>MDYKDDDDKLAAANSSIDLISTSLYKKAGFRTMTSIHFVVHPLPGTEDQLNDRLREVSEKLNKYNLNSHPPLNVLEQATIKQCVVGPNHAAFLLEDGRVCRIGFSVQPDRLELGKPDNNDGSKLNSNSGAGRTSRPGRTSDSPWFLSGSETLGRLAGNTLGSRWSSGVGGSGGGSSGRSSAGARDSRRQTRVIRTGRDRGSGLLGSQPQPVIPASVIPEELISQAQVVLQGKSRSVIIRELQRTNLDVNLAVNNLLSRDDEDGDDGDDTASESYLPGEDLMSLLDADIHSAHPSVIIDADAMFSEDISYFGYPSFRRSSLSRLGSSRVLLLPLERDSELLRERESVLRLRERRWLDGASFDNERGSTSKEGEPNLDKKNTPVQSPVSLGEDLQWWPDKDGTKFICIGALYSELLAVSSKGELYQWKWSESEPYRNAQNPSLHHPRATFLGLTNEKIVLLSANSIRATVATENNKVATWVDETLSSVASKLEHTAQTYSELQGERIVSLHCCALYTCAQLENSLYWWGVVPFSQRKKMLEKARAKNKKPKSSAGISSMPNITVGTQVCLRNNPLYHAGAVAFSISAGIPKVGVLMESVWNMNDSCRFQLRSPESLKNMEKASKTTEAKPESKQEPVKTEMGPPPSPASTCSDASSIASSASMPYKRRRSTPAPKEEEKVNEEQWSLREVVFVEDVKNVPVGKVLKVDGAYVAVKFPGTSSNTNCQNSSGPDADPSSLLQDCRLLRIDELQVVKTGGTPKVPDCFQRTPKKLCIPEKTEILAVNVDSKGVHAVLKTGNWVRYCIFDLATGKAEQENNFPTSSIAFLGQNERNVAIFTAGQESPIILRDGNGTIYPMAKDCMGGIRDPDWLDLPPISSLGMGVHSLINLPANSTIKKKAAVIIMAVEKQTLMQHILRCDYEACRQYLMNLEQAVVLEQNLQMLQTFISHRCDGNRNILHACVSVCFPTSNKETKEEEEAERSERNTFAERLSAVEAIANAISVVSSNGPGNRAGSSSSRSLRLREMMRRSLRAAGLGRHEAGASSSDHQDPVSPPIAPPSWVPDPPAMDPDGDIDFILAPAVGSLTTAATGTGQGPSTSTIPGPSTEPSVVESKDRKANAHFILKLLCDSVVLQPYLRELLSAKDARGMTPFMSAVSGRAYPAAITILETAQKIAKAEISSSEKEEDVFMGMVCPSGTNPDDSPLYVLCCNDTCSFTWTGAEHINQDIFECRTCGLLESLCCCTECARVCHKGHDCKLKRTSPTAYCDCWEKCKCKTLIAGQKSARLDLLYRLLTATNLVTLPNSRGEHLLLFLVQTVARQTVEHCQYRPPRIREDRNRKTASPEDSDMPDHDLEPPRFAQLALERVLQDWNALKSMIMFGSQENKDPLSASSRIGHLLPEEQVYLNQQSGTIRLDCFTHCLIVKCTADILLLDTLLGTLVKELQNKYTPGRREEAIAVTMRFLRSVARVFVILSVEMASSKKKNNFIPQPIGKCKRVFQALLPYAVEELCNVAESLIVPVRMGIARPTAPFTLASTSIDAMQGSEELFSVEPLPPRPSSDQSSSSSQSQSSYIIRNPQQRRISQSQPVRGRDEEQDDIVSADVEEVEVVEGVAGEEDHHDEQEEHGEENAEAEGQHDEHDEDGSDMELDLLAAAETESDSESNHSNQDNASGRRSVVTAATAGSEAGASSVPAFFSEDDSQSNDSSDSDSSSSQSDDIEQETFMLDEPLERTTNSSHANGAAQAPRSMQWAVRNTQHQRAASTAPSSTSTPAASSAGLIYIDPSNLRRSGTISTSAAAAAAALEASNASSYLTSASSLARAYSIVIRQISDLMGLIPKYNHLVYSQIPAAVKLTYQDAVNLQNYVEEKLIPTWNWMVSIMDSTEAQLRYGSALASAGDPGHPNHPLHASQNSARRERMTAREEASLRTLEGRRRATLLSARQGMMSARGDFLNYALSLMRSHNDEHSDVLPVLDVCSLKHVAYVFQALIYWIKAMNQQTTLDTPQLERKRTRELLELGIDNEDSEHENDDDTNQSATLNDKDDDSLPAETGQNHPFFRRSDSMTFLGCIPPNPFEVPLAEAIPLADQPHLLQPNARKEDLFGRPSQGLYSSSASSGKCLMEVTVDRNCLEVLPTKMSYAANLKNVMNMQNRQKKEGEEQPVLPEETESSKPGPSAHDLAAQLKSSLLAEIGLTESEGPPLTSFRPQCSFMGMVISHDMLLGRWRLSLELFGRVFMEDVGAEPGSILTELGGFEVKESKFRREMEKLRNQQSRDLSLEVDRDRDLLIQQTMRQLNNHFGRRCATTPMAVHRVKVTFKDEPGEGSGVARSFYTAIAQAFLSNEKLPNLECIQNANKGTHTSLMQRLRNRGERDREREREREMRRSSGLRAGSRRDRDRDFRRQLSIDTRPFRPASEGNPSDDPEPLPAHRQALGERLYPRVQAMQPAFASKITGMLLELSPAQLLLLLASEDSLRARVDEAMELIIAHGRENGADSILDLGLVDSSEKVQQENRKRHGSSRSVVDMDLDDTDDGDDNAPLFYQPGKRGFYTPRPGKNTEARLNCFRNIGRILGLCLLQNELCPITLNRHVIKVLLGRKVNWHDFAFFDPVMYESLRQLILASQSSDADAVFSAMDLAFAIDLCKEEGGGQVELIPNGVNIPVTPQNVYEYVRKYAEHRMLVVAEQPLHAMRKGLLDVLPKNSLEDLTAEDFRLLVNGCGEVNVQMLISFTSFNDESGENAEKLLQFKRWFWSIVEKMSMTERQDLVYFWTSSPSLPASEEGFQPMPSITIRPPDDQHLPTANTCISRLYVPLYSSKQILKQKLLLAIKTKNFGFV[2x]

Here, we used genetic screens to identify the HECT-family protein ubiquitin protein ligase E3 component n-recognin 5 (UBR5) as the E3 ubiquitin ligase that governs agonist-induced degradation of numerous NRs and characterized these interactions biochemically and structurally. We next structurally interrogated functional domains in the context of full-length UBR5, which is expressed predominantly as a 310 kDa polypeptide product in humans. The N-terminal region of UBR5 arranges into a seven-bladed β-propeller, which shows weak homology to a regulator of chromosome condensation 1 (RCC1)-like domain (RLD). Following the RLD, a large helical region forms the core scaffold of UBR5.

To unambiguously assign this weaker density, we expressed and purified a mutant version of UBR5 lacking residues 522–720 (UBR5Δtandem), which in SEC-MALS was consistent with a dimer (648 kDa). In cryo-EM analysis the dimeric UBR5Δtandem is held together solely by the rigid interface in the central helical bundle (bottom, S4A, and S4B). Reduced orientation bias of the dimeric UBR5 particles allowed us to generate an improved map at ~3.4 Å resolution. One dimerization interface is maintained through a large central helical bundle (residues 1,350–2,110), which is among the highest resolution regions of the EM map. The insertion following the 2nd blade is largely unobserved in our EM reconstructions and is predicted to be unstructured, except for the 50 amino acid region that folds into a classical UBA domain. The other insertion between the 5th and 6th blades forms the aforementioned dimerization interface (residues 522–720). The eponymous UBR domain, a small motif containing three zinc ions, protrudes from this central region and is also clearly observed in the cryo-EM density map. As in other HECT-family ubiquitin ligases, the catalytic HECT domain of UBR5 is found at its extreme C-terminus. We observe an additional density from an upstream region (residues 2,022–2,067) wedged into a hydrophobic surface on the HECT N-lobe, promoting a predominant L-shaped conformation of the HECT domains. This region, which we refer to as the “wedge”, is poised to influence conformational dynamics of the HECT domain over a catalytic cycle and also scores as one of the top hits in our tiling screen (residue 2,050). The EM density maps have been deposited at the Electron Microscopy Data Bank database with accession code EMD-17539 (UBR5 dimer), EMD-17540 (UBR5 tetramer), and EMD-17542 (negative stain map of UBR5 dimer with RARA/RXRA).>IKDPQTGAPVPLRALINNVSGYVIKTEMYTEVKNAKGEWVFKSLGKPGSMHLRPIATPYPVKEWLQPKRYKAHLMGTTYVYDFPELFRQASSSQWKNFSADVKLTDDFFISNELIEDENGELTEVEREPGANAIGMVAFKITVKTPEYPRGRQFVVVANDITFKIGSFGPQEDEFFNKVTEYARKRGIPRIYLAANSGARIGMAEEIVPLFQVAWNDAANPDKGFQYLYLTSEGMETLKKFDKENSVLTERTVINGEERFVIKTIIGSEDGLGVECLRGSGLIAGATSRAYHDIFTITLVTCRSVGIGAYLVRLGQRAIQVEGQPIILTGAPAIN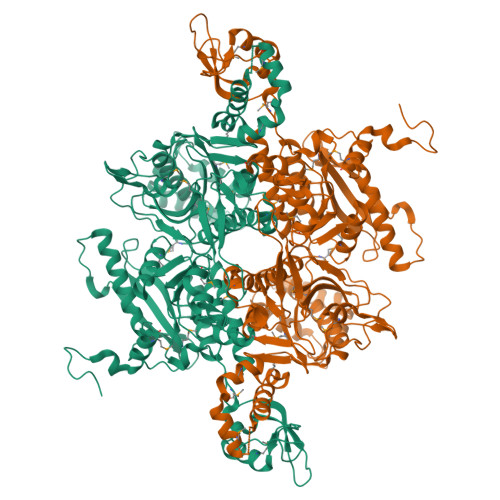KMLGREVYTSNLQLGGTQIMYNNGVSHLTAVDDLAGVEKIVEWMSYVPAKRNMPVPILETKDTWDRPVDFTPTNDETYDVRWMIEGRETESGFEYGLFDKGSFFETLSGWAKGVVVGRARLGGIPLGVIGVETRTVENLIPADPANPNSAETLIQEPGQVWHPNSAFKTAQAINDFNNGEQLPMMILANWRGFSGGQRDMFNEVLKYGSFIVDALVDYKQPIIIYIPPTGELRGGSWVVVDPTINADQMEMYADVNARAGVLEPQGMVGIKFRREKLLDTMNRLDDKYRELRSQLSNKSLAPEVHQQISKQLADRERELLPIYGQISLQFADLHDRSSRMVAKGVISKELEWTEARRFFFWRLRRRLNEEYLIKRLSHQVGEASRLEKIARIRSWYPASVDHEDDRQVATWIEENYKTLDDKLKGLKLESFAQDLAKKIRSDHDNAIDGLSEVIKMLSTDDKEKLLKTLK[3x]> STAGKVIKCKAAVLWEEKKPFSIEEVEVAPPKAHEVRIKMVATGICRSDDHVVSGTLVTPLPVIAGHEAAGIVESIGEGVTTVRPGDKVIPLFTPQCGKCRVCKHPEGNFCLKNDLSMPRGTMQDGTSRFTCRGKPIHHFLGTSTFSQYTVVD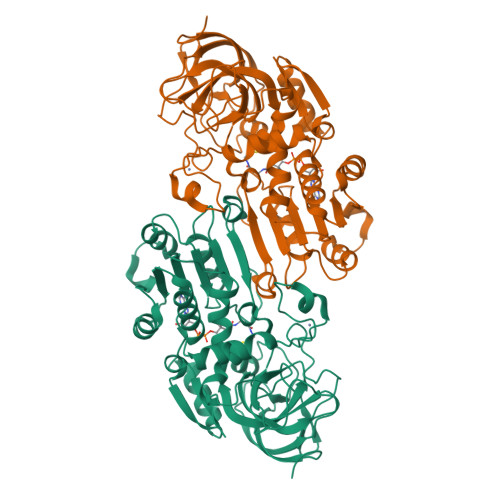EISVAKIDAASPLEKVCLIGCGFSTGYGSAVKVAKVTQGSTCAVFGLGGVGLSVIMGCKAAGAARIIGVDINKDKFAKAKEVGATECVNPQDYKKPIQEVLTEMSNGGVDFSFNVIGRLDTMVTALSCCQEAYGVSVIVGVPPDSQNLSMNPMLLLSGRTWKGAIFGGFKSKDSVPKLVADFMAKKFALDPLITHVLPFEKINEGFDLLRSGESIRTILTF>ASWSHPQFEKIEGRRDRGPEFLAKQYKNLVNGEWKLSENEITIYAPATGEELGSVPAMTQAEVDAVYASAKKALSDWRTLSYVERAAYLHKAADILVRDAEKIGAILSKEVAKGHKAAVSEVIRTAEIINYAAEEGLRMEGEVLEGGSFEAASKKKIAIVRREPVGLVLAISPFNYPVNLAGSKIAPALIAGNVVALKPPTQGSISGLLLAEAFAEAGIPAGVFNTITGRGSVIGDYIVEHEAVNFINFTGSTPIGEGIGKLAGMRPIML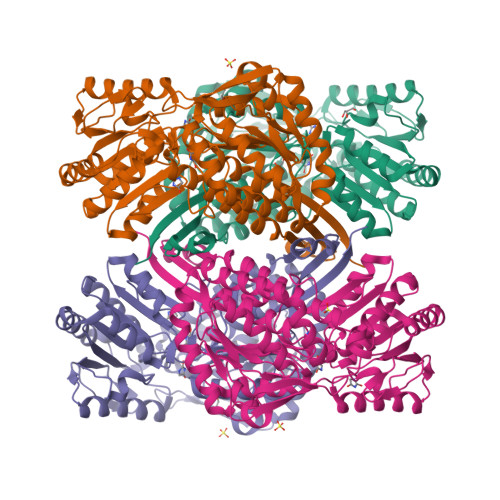ELGGKDSAIVLEDADLALAAKNIVAGAFGYSGQRSTAVKRVLVMDKVADQLAAEIKTLVEKLSVGMPEDDADITPLIDTSAADFVEGLIKDATDKGATALTAFNREGNLISPVLFDHVTTDMRLAWEEPFGPVLPIIRVTTVEEAIKISNESEYGLQASIFTTNFPKAFGIAEQLEVGTVHLNNKTQRGTDNFPFLGAKKSGAGVQGVKYSIEAMTTVKSVVFDIQ[8x]> RSHHHHHHGCLTQLYENAFFRGGDVASMYTPNAQYCQMRCTFHPRCLLFSFLPASSINDMEKRFGCFLKDSVTGTLPKVHRTGAVSGHSLKQCGHQISACHRDIYKGVDMRGVNFNVSKVSSVEECQKRCTNNIRCQFFSYATQTFHKAEYRNNCLLKYSPGGTPTAIKVLSNVESGFSLKPCALSEIGCHMNIFQHLAFSDVDVARVLTPDAFVCRTICTYHPNCLFFTFYTNVWKIESQRNVCLLKTSESGTPSSSTPQENTISGYSLLTCKRTLPEPCHSKIYPGVDFGGEELNVTFVKGVNVCQETCTKMIRCQFFTYSLLPEDCKAEACKCFLRLSMDGSPTRIAYGTQGSSGYSLRLCNTGDNSVCTTKTSTRIVGGTQSSWGEWPWQVSLQVKLTAQRHLCGGSLIGHQWVLTAAHCFDGLPLQDVWRIYSGILQLSDITKDTPFSQIKEIIIHQNYKVSEGNHDIALIKLQAPLQYTEFQKPICLPSKGDTSTIYTNCWVTGWGFSAEAGEIQNILQKVNIPLVTNEECQKRYQDYKITQRMVCAGYKEGGKDACKGDAGGPLVCKHNGMWRLVGITSWGEGCARREQPGVYTKVAEYMDWILEKTQSSDGKAQMQSPA

The regulation of extracellular proteolysis is critical to blood hemostasis and innate immunity and proteases plasma prekallikrein (PK), and coagulation factors XII (FXII) and XI (FXI) act as master regulators of several cascades including coagulation, fibrinolysis, complement activation, and inflammation 1, 2, 3, 4. PK and FXI are homologous and share 58% amino acid sequence identity with the unique feature of four tandem repeats of 90 amino acid apple domains at the N‐terminus, which harbor exosites for substrates, cofactors, and receptors 18. Factor XI is a disulfide‐linked dimer whereas PK is a monomer 20, 21. Factor XIIa recognizes and cleaves both PK and FXI but it is unknown which of the apple domains is critical for these interactions or the molecular basis of the reciprocal cleavage of the FXII zymogen by PKa.

To determine a full‐length PKa structure recombinant optimized PK active site mutant S559A was activated by proteolytic cleavage of the activation loop Arg371‐Ile372 using FXIIa. PKa crystallized in the presence of inhibitor benzamidine and the structure was determined to 1.3 Å resolution. The PKa protease structure consists of two β‐barrels and the benzamidine inhibitor is observed bound in the active site S1 pocket with the Ile372 residue from the activation loop forming the characteristic electrostatic interaction with Asp558. The full‐length structure defines the interactions formed between the PKa protease domain and the apple domains whereby two extended loops “latch” on to the apple domains with specific interactions shown in Fig. 1C. Residues 476 to 484 form a latch loop1 and residues 566 to 570 comprise latch loop2. Latch loop1 contains a central β‐hairpin that inserts the salt bridged residues Glu478‐Lys481 into a pocket at the center of the apple domain disc where Glu478 forms hydrogen bonds with Arg267 and Ser90. Latch loop2 adopts an extended β‐hairpin and on its tip residue Lys566 forms a salt bridge to Asp95 from the apple 2 domain and Gly569 in latch loop2 forms a hydrogen bond to Gln26 from the apple 1 domain topside α‐helix. An alternate conformation occurs in the apple 4 domain where an internal Cys321‐Cys326 disulfide distinguishes PK as a monomer precluding formation of the extensive disulfide‐linked dimer interface observed in FXI 19. A comparison of the full‐length structures of PKa with the FXI zymogen revealed a large unexpected conformational 180° rotational rearrangement of the intact apple domain disc relative to the protease domain. The PKa latch loop1 is a key pivot point for this relative rotation as it contains the Cys364‐Cys484 disulfide which anchors the protease domain to the apple domains after cleavage of the Arg371‐Ile373 peptide bond in the activation loop.> RNILRNDEGLYGGQSLDVNPYHFIMQEDCNLVLYDHSTSVWASNTGILGKKGCRAVLQSDGNFVVYDAEGRSLWASHSVRGNGNYVLVLQEDGNVVIYRSDIWSTN;> RNILTNDEGLYGGQSLDVNPYHLIMQEDCNLVLYDHSTAVWSSNTDIPGKKGCKAVLQSDGNFVVYDAEGASLWASHSVRGNGNYVLVLQEDGNVVIYRSDIWSTNTYR;> RNILTNDEGLYAGQSLDVNPYHFIMQEDCNLVLYDHSTSVWASNTGILGKKGCKAVLQADGNFVVYDAEGRSLWASHSVRGNGNYVLVLQEDGNVVIYGSDIWSTN;> RNILTNDEGLYAGQSLDVNPYHLIMQEDCNLVLYDHSTAVWSSNTDIPGKKGCKAVLQSD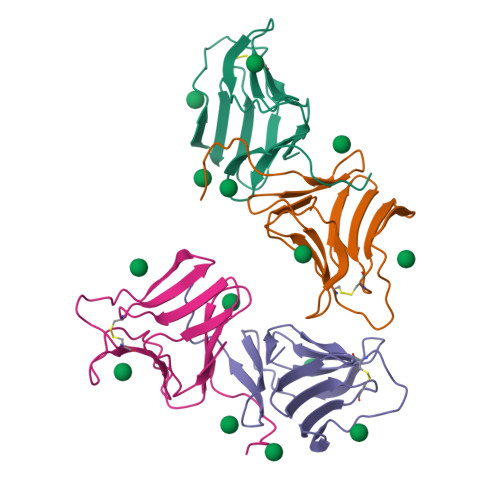GNFVVYDAEGASLWASHSVRGNGNYVLVLQEDGNVVIYGSDIWSTNTYK>MSDKLPYKVADIGLAAWGRKALDIAENEMPGLMRMRERYSASKPLKGARIAGCLHMTVETAVLIETLVTLGAEVQWSSCNIFSTQNHAAAAIAKAGIPVYAWKGETDEEYLWCIEQTLYFKDGPLNMILDDGGDLTNLIHTKYPQLLPGIRGISEETTTGVHNLYKMMANGILKVPAINVNDSVTKSKFDNLYGCRESLIDGIKRATDVMIAGKVAVVAGYGDVGKGCAQALRGFGARVIITEIDPINALQAAMEGYEVTTMDEACQEGNIFVTTTGCIDIILGRHFEQMKDDAIVCNIGHFDVEIDVKWLNENAVEKVNIKPQVDRYRLKNGRRIILLAEGRLVNLGCAMGHPSFVMSNSFTNQVMAQIELWTHPDKYPVGVHFLP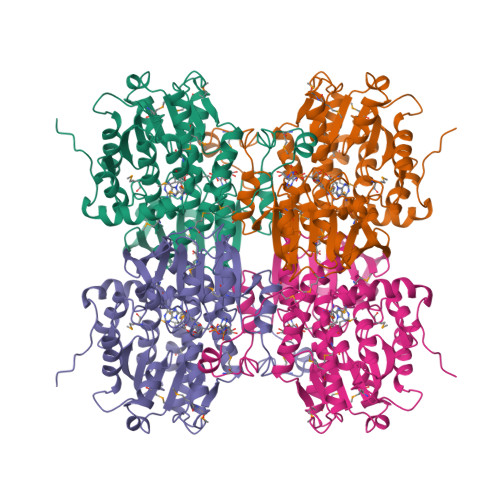KKLDEAVAEAHLGKLNVKLTKLTEKQAQYLGMSCDGPFKPDHYRY[2x]2'-(3-IODOPHENYL)-5-(4-METHYL-1-PIPERAZINYL)-2,5'-BI-BENZIMIDAZOLE | C25 H24 I N6 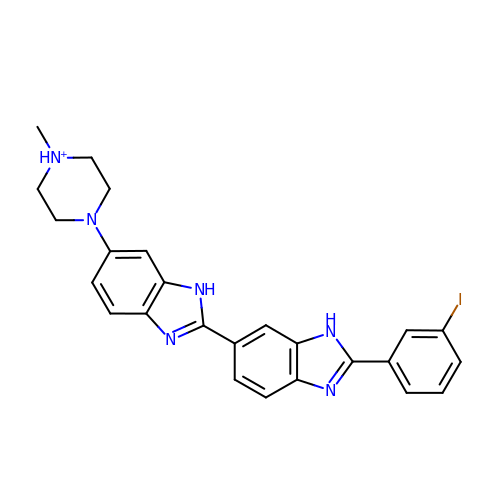| ZEXOKHKEQNNOBG-UHFFFAOYSA-O>MPKIYTKTGDKGFSSTFTGERRPKDDQVFEAVGTTDELSSAIGFALELVTEKGHTFAEELQKIQCTLQDVGSALATPCSSAREAHLKYTTFKAGPILELEQWIDKYTSQLPPLTAFILPSGGKISSALH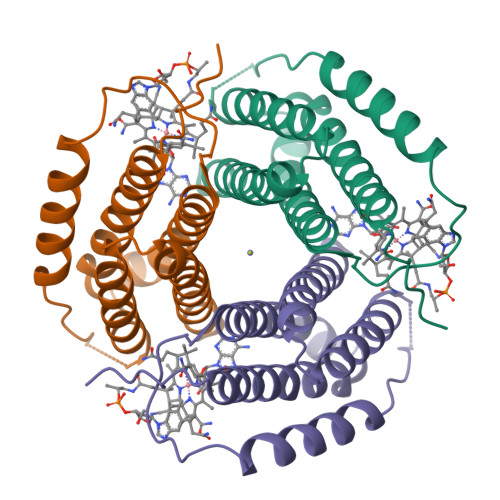FCRAVCRRAKRRVVPLVQMGETDANVAKFLNRLSDYLFTLARYAAMKEGNQEKIYMKNDPSAESEGL[4x]>MAEIGTGFPFDPHYVEVLGERMHYVDVGPRDGTPVLFLHGNPTSSYVWRNIIPHVAPTHRCIAPDLIGMGKSDKPDLGYFFDDHVRFMDAFIEALGLEEVVLVIHDWGSALGFHWAKRNPERVKGIAFMEFIRPIPTWDEWPEFARETFQAFRTTDVGRKLIIDQNVFIEGTLPMGVVRPLTEVEMDHYREPFLNPVDREPLWRFPNELPIAGEPANIVALVEEYMDWLHQSPVPKLLFWGTPGVLIPPAEAARLAKSLPNCKAVDIGPGLNLLQEDNPDLIGSEIARWLSTLEISGHHHHHH[2x]

Here we present a GSH-sensing platform for live-cell imaging, termed targetable ratiometric quantitative GSH (TRaQ-G). We hypothesized that a SiR dye in a spirocyclic form would be non-reactive against GSH, but it could isomerize to its zwitterionic form upon binding to the self-labelling protein HaloTag (HT), switching both its fluorescence and reactivity against GSH from an ‘off’ to an ‘on’ state. In conclusion, we have designed, synthesized and validated a new ratiometric GSH sensor, TRaQ-G, which only becomes reactive in the organelle of interest. This sensor is based on binding of a spirocyclic SiR ligand to HT, which induces isomerization to the GSH-sensitive and fluorescent zwitterionic form. We conducted X-ray diffraction experiments and MD simulations for structural elucidation of the different TRaQ-G adducts to gain mechanistic insight into the varying GSH sensitivities of the molecules.

We thus refer to the HT-bound carboxylic-acid derivative as TRaQ-G-ctrl, whereas the cyanamide derivative is hereafter called TRaQ-G. GSH titration experiments revealed that, whereas the HT-bound carboxylic-acid derivative was completely insensitive to GSH, the cyanamide ligand bound to HT responded to GSH in the physiologically relevant range of concentrations (~1–20 mM). To understand the difference in reactivity between TRaQ-G-ctrl and TRaQ-G, we analysed the structure of both conjugates by X-ray diffraction. Whereas the spirocyclic form binds similarly to Me–TRaQ-G and TRaQ-G-ctrl, the zwitterionic form occupies an alternative pocket. MD simulations using the spirocyclic form as a starting point suggest that the side chain of residue F144 must rotate to allow for the ligand to occupy the alternative pocket and thus switch to its zwitterionic form. Using MD simulations starting from the zwitterionic structure, we found that the structure rapidly relaxes to a stable conformation in which the cyanamide forms a persistent hydrogen bond with the backbone carbonyl of residue P243. This interaction exposes the opposite face of the SiR dye to the solvent, allowing for GSH attack (Fig. 2d(bottom right)), explaining the reactivity observed in titration experiments. Instead, we focused on TRaQ-G, the ligand of which undergoes fluorescence and reactivity turn-on upon binding to HT. Once bound to HT, the strong fluorescence of the TRaQ-G ligand decreases upon reaction with GSH.The THDI mediates binding of Myo3 to its cargo protein Espin1 (Ectoplasmic specialization protein 1) and allows Myo3 to transport Espin1 to the tips of actin bundle-based structures such as filopodia and stereocilia. Espin1 is the longest isoform in the family and contains a stretch of ankyrin repeats (AR) in its N-terminus. Here, we discover that both Myo3a and Myo3b contain two highly similar repeat sequences in their THDI region, each capable of independently binding to Espin1-AR with high affinity. The high resolution crystal structures of each of the two binding sequences from Myo3b in complex with Espin1-AR not only reveal the molecular basis governing the specific interaction between Myo3 and Espin1, but also allow us to discern the Myo3-mediated release of the auto-inhibition mechanism of Espin1.

To understand the molecular basis of the Espin1/Myo3 interaction, we solved the crystal structure of the Espin1-AR/Myo3b-ARB1 complex at 1.65 Å resolution. The structure revealed that Espin1-AR contains 10 ANK repeats, instead of 8 as predicted earlier. The 10 ANK repeats form a left-handed superhelix with the αA helices forming the inner groove and the αB helices forming the outer surface. Clear additional electron densities lining the inner groove of the ANK repeats allowed us to build the bound Myo3b-ARB1 peptide model with high confidence. The ARB1 binds to Espin1-AR in an antiparallel manner, similar to the binding mode between ANK repeats from Ankyrin R/B/G and their targets as well as between ANKRA2/RFXANK and their targets, suggesting that elongated inner grooves are common target binding sites of ANK repeats in general. The ARB1 spans nearly the entire inner groove, covering ~1230 Å2 of solvent accessible area. The N-terminal of ARB1 adopts an extended structure and binds to the C-terminal of Espin1-AR. The C-terminal of ARB1 forms an α-helix and binds to the N-terminal half of Espin1-AR. The first binding site is formed by the repeats 2–4 of Espin1-AR and binds to the C-terminal α-helix of ARB1 (Figure 3A1). Two absolutely conserved tyrosine residues (Tyr1267ARB1 and Tyr1268ARB1, the double tyrosine (‘YY’) motif; Figure 3B) and Leu1271ARB1 in the next turn insert into the hydrophobic pocket in the N-terminal of Espin1-AR (Figure 3A1). The two highly conserved Arg residues at the beginning of Myo3b-ARB1 (Arg1251ARB1 and Arg1252ARB1) insert into the negatively charged pocket (Figure 3A3).

>AMALEQALQAARRGDLDVLRSLHAAGLLGPSLRDSLDALPVHHAARSGKLHCLRYLVEEVALPAVSRARNGATPAHDAAATGYLSCLQWLLTQGGCRVQEKDNSGATVLHLAARFGHPDVVKWLLYQGGANSAITTDTGALPIHYAAAKGDLPSLKLLVGHYPEGVNAQTNNGATPLYLACQEGHLEVTKYLVQECSADPHLRAQDGMTPLHAAAQMGHNPVLVWLVSFADVSFSEQDHDGATAMHFAASRGHTKVLSWLLLHGAEISQDLWGGTPLHDAAENGELECCQILAVNGAGLDVRDHDGYTAADLAEFNGHTHCSRYLRTVQTLSLEHRVLSRDQSMDLEAKQLDS[2x];>QKQRAPRRRCQQPKMLSSPEDTMYYNQLNGTLEYQG[2x]>[12x]TLSRDDAAQVAKVLSE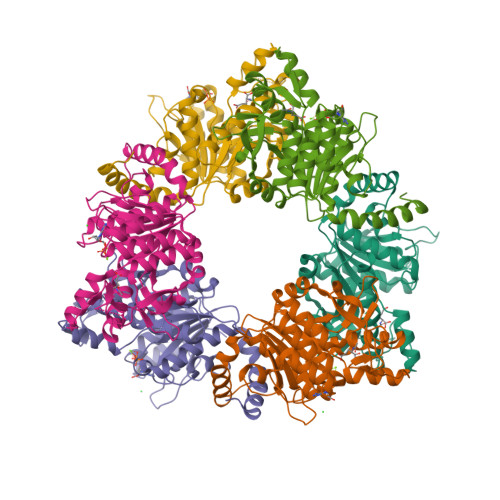ALPYIRRFVGKTLVIKYGGNAMESEELKAGFARDVVLMKAVGINPVVVHGGGPQIGDLLKRLSIESHFIDGMRVTDAATMDVVEMVLGGQVNKDIVNLINRHGGSAIGLTGKDAELIRAKKLTVTRQTPEMTKPEIIDIGHVGEVTGVNVGLLNMLVKGDFIPVIAPIGVGSNGESYNINADLVAGKVAEALKAEKLMLLTNIAGLMDKQGQVLTGLSTEQVNELIADGTIYGGMLPKIRCALEAVQGGVTSAHIIDGRVPNAVLLEIFTDSGVGTLISNRKRH~{N}-(3-methoxyphenyl)-4-methyl-3-[(1-methyl-6-pyridin-3-yl-pyrazolo[3,4-d]pyrimidin-4-yl)amino]benzamide 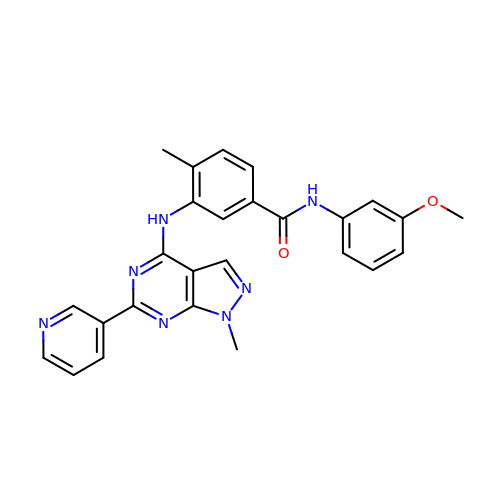| C26 H23 N7 O2 | AWTFDMFFAXABDI-UHFFFAOYSA-N> XVVFAF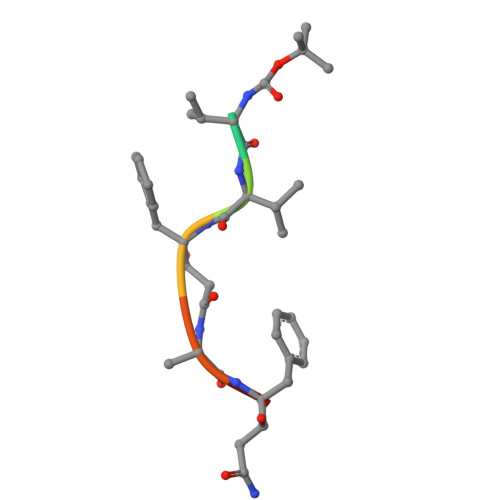A> RSVAHLFIDETSSEVLDELYRVSKEYTHSRPQAQRVIKDLIKVAIKVAVLHRNGSFGPSELALATRF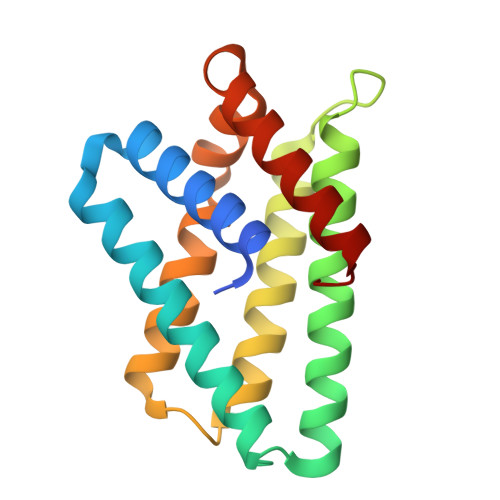RQKLRQGAMTALSFGEVDFTFEAAVLAGLLTECRDVLLELVEHHLTPKSHGRIRHVFDHFSDPGLLTALYGPDFTQHLGKICDGLRKLLDEGKL>[4x]STPSIVIASAARTAVGSFNGAFANTPAHELGATVISAVLERAG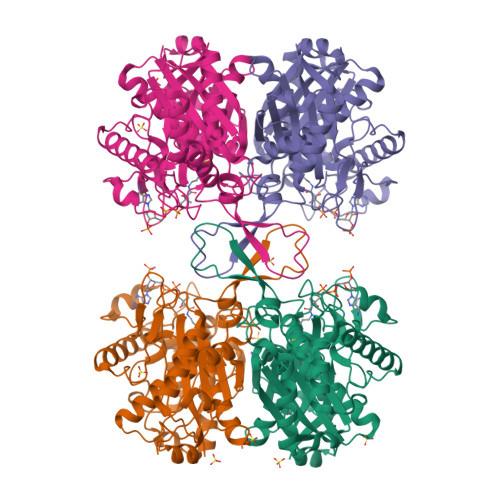VAAGEVNEVILGQVLPAGEGQNPARQAAMKAGVPQEATAWGMNQLCGSGLRAVALGMQQIATGDASIIVAGGMESMSMAPHCAHLRGGVKMGDFKMIDTMIKDGLTDAFYGYHMGTTAENVAKQWQLSRDEQDAFAVASQNKAEAAQKDGRFKDEIVPFIVKGRKGDITVDADEYIRHGATLDSMAKLRPAFDKEGTVTAGNASGLNDGAAAALLMSEAEASRRGIQPLGRIVSWATVGVDPKVMGTGPIPASRKALERAGWKIGDLDLVEADEAFAAQACAVNKDLGWDPSIVNVNGGAIAIGHPIGASGARILNTLLFEMKRRGARKGLATLCIGGGMGVAMCIESL>[2x]MEKKTIVLGVIGSDCHAVGNKILDHAFTNAGFNVVNIGVLSPQENFIKAAIETKADAILVSSLYGQGEIDCKGLRQKCDEAGLEGILLYVGGNIVVGKQHWPDVEKRFKDMGYDRVYAPGTPPEVGIADLKKDLNIE;>[2x]MELKNKKWTDEEFHKQREEVLQQWPTGKEVDLQEAVDYLKKIPAEKNFAEKLVLAKKKGITMAQPRAGVALLDEHIELLRYLQDEGGADFLPSTIDAYTRQNRYDECENGIKESEKAGRSLLNGFPGVNHGVKGCRKVLEAVNLPLQARHGTPDSRLLA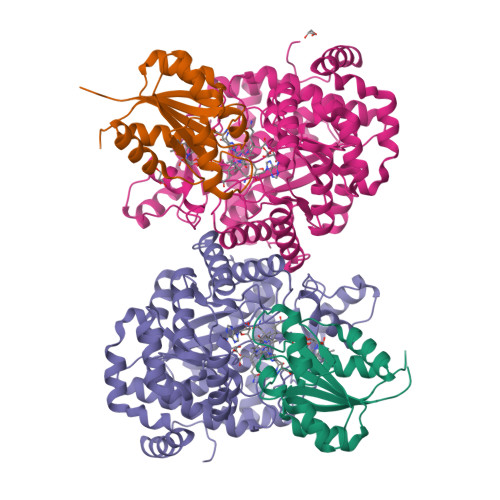EIIHAGGWTSNEGGGISYNVPYAKNVTIEKSLLDWQYCDRLVGFYEEQGVHINREPFGPLTGTLVPPSMSNAVGITEALLAAEQGVKNITVGYGECGNMIQDIAALRCLEEQTNEYLKAYGYNDVFVTTVFHQWMGGFPQDESKAFGVIVTATTIAALAGATKVIVKTPHEAIGIPTKEANAAGIKATKMALNMLEGQRMPMSKELETEMAVIKAETKCILDKMFELGKGDLAIGTVKAFETGVMDIPFGPSKYNAGKMMPVRDNLGCVRYLEFGNVPFTEEIKNYNRERLQERAKFEGRDVSFQMVIDDIFAVGKGRLIGRPE> XNRVFAEYPDHIQDYFK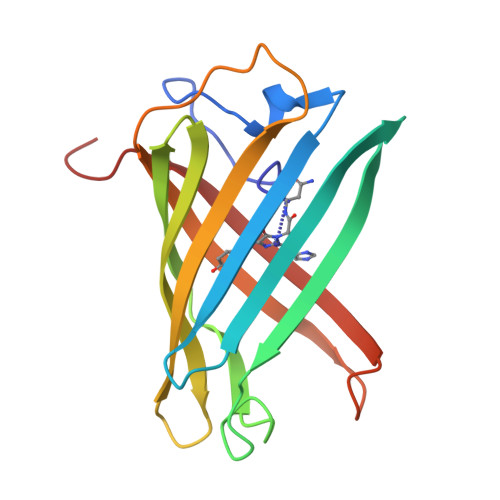QSFPKGYSWERSLTFEDGGICIARNDITMEGDTFYNKVRFHGVNFPANGPVMQKKTLKWEPSTEKMYVRDGVLTGDITMALLLEGNAHYRCDFRTTYKAKEKGVKLPGYHFVDHCIEILSHDKDYNKVKLYEHAVAHSGLPD>MVRGRVPQIQARQINIFGIVQGVGFRPFVFNIAQKYNLKGIVYNNSSGLYIEVEGEEKDIEAFIREIKENPPSLSVIDEIQVREVEVKEYKDFKIVGSKEDGGFVPVSPDMGVCEDCLRELKDPKDRRYRYPFINCTNCGPRFSIIEDIPYDRAKTSMKVFPMCEKCSREYHDPHDRRFHAQPVACFDCGPSLSFVGEGCFDDEIKCVAKALKEGKIVAIKGIGGFHLAVNALDDEAVATLRRRK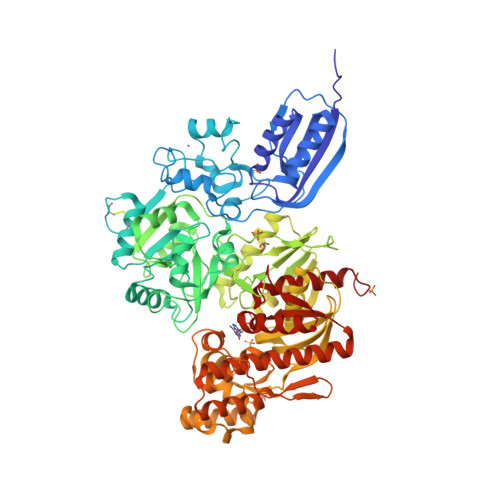KRYGKPFAVMMRDVEEVKKYCIVSPEEERLLLSQRRPIVLLKKKGEKLAKGIADDLDTLGVMLPYAPIHYLLMEEIDFPIVMTSGNVSEEPICKDNEEALEKLKDIADVFLLNNRDIVNRIDDSVTSFNAGAERIIRRARGYAPQPILLKKEVKASILAVGGFYKNTFCMTKGHYAFISHHIGDLDNEKAFNYYIEQIERYKKLFRVDPEVVAHDMHKGYLSTQYAKSLDLPKIEVQHHHAHIASCMAEHNLDEKVIGIAYDGTGYGTDGNVWGAEILVCDLKSFERIAHLKYKPLPGNELAIKKIYRTALGFIFDNISFYKNFVEQVDSRELDIILKQIDRKINTAYVSSMGRFFDAVAALIGVRKEVLFEGQAAMELESLMAESEEYYEYEILKEDRYVIDPELILRQIYEDYMKGFEKSYISAKFHNTVVNFTYDLANLIRKETGINKVVLSGGSFQNRYLLRRLIEKLSLSGFEVYSNSKVPCNDGGISLGQAVIANKILEGSAWSHPQFEK[2x]> ALPQTVRIGTDTTYAPFSSKDAKGEFIGFDIDLGNEMCKRMQVKCTWVASDFDALIPSLKAKKIDAIISSLAITDKRQQEIAFSDKLYAADSRLIAAKGSPIQPTLESLKGKHVGVLQGSTQEAYANDNWRTKGVDVVAYA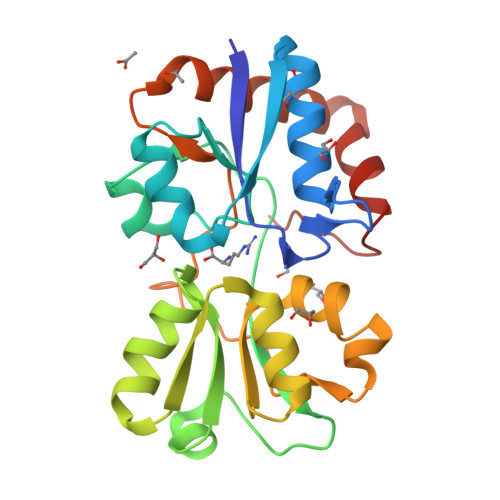NQDLIYSDLTAGRLDAALQDEVAASEGFLKQPAGKEYAFAGPSVKDKKYFGDGTGVGLRKDDTELKAAFDKALTELRQDGTYDKMAKKYFDFNVYGD> MFYIDNDSGVTVMPPVSAQRSAIVRWFSEGDGNNVITWPGMDWFNIVQAELLNTLEEAGIQPDKTKLNQLALSIKAIMSNNALLIKNNLSEIKTAGASAQRTARENLDIYDASLNKKGLVQLTSATDSPSETLAATAKAVKIAMDNANARLAKDRNGADIPNKPLFIQNLGLQETVNRARNAVQKNGDTLSGGLTFENDSILAWIRNTDWAKIGFKNDADSDTDSYMWFETGDNGNEYFKWRSKQSTTTKDLMNLKWDALSVLVNAIVNGEVISKSANGLRIAYGNYGFFIRNDGSNTYFMLTNSGDNMGTYNGLRPLWINNATGAVSMGRGLNVSGDTLSDRFAINSSNGMWIQMRDNNAIFGKNIVNTDSAQALLRQNHADRKFMIGGLGNKQFGIYMINNSRTANGTDGQAYMDNNGNWLCGAQVIPGNYANFDSRYVRDVRLGTQSLTGGLSRDYKAPSGHVITGFHTNGDWEMQGGDDKVYIRPVQKNINGTWYNVASA;> MMHLKNIKSENPKTKEQYQLTKNFD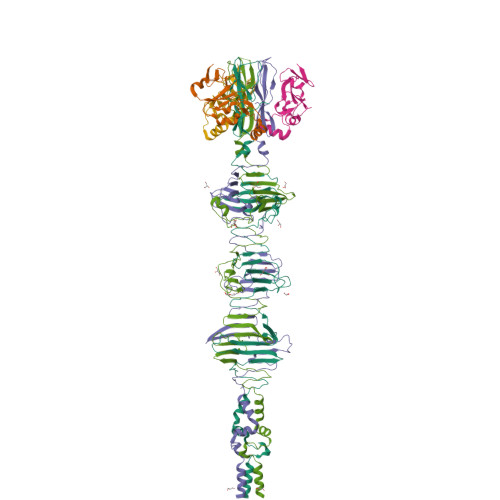VIWLWSEDGKNWYEEVNNFQDDTIKIVYDENNIIVAITKDASTLNPEGFSVVEIPDITANRRADDSGKWMFKDGAVVKRIYTADEQQQQAESQKAALLSEAESVIQPLERAVRLNMATDEERARLESWERYSVLVSRVDTANPEWPQKPE> GPLGSVVRAKFNFQQTNEDE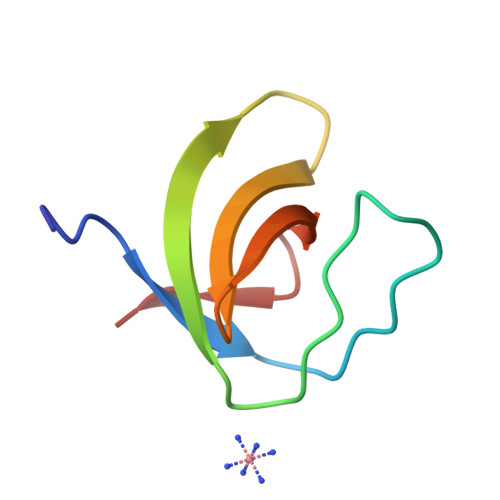LSFSKGDVIHVTRVEEGGWWEGTHNGRTGWFPSNYVREI>GMSRDRLYTWAGLWRSPSSSWEALRLEDDQAESQLRAPDERSGLPYQLDYRLRWDADWHLREAVFHVESETGVRKLHLLADGRGHWQDGDGEALPAFDGCLDIDIWPSPFTNTFPIRRLGLADGQRAEIRALYIEA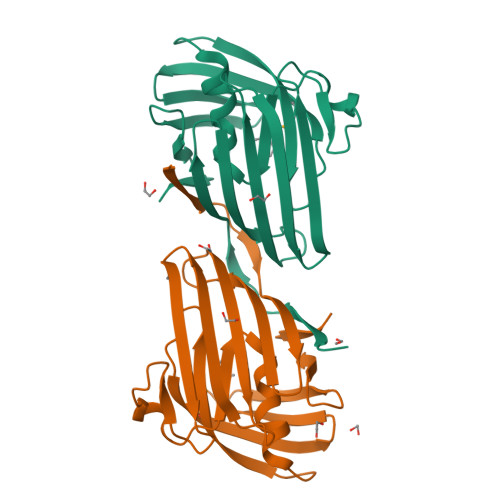PALEPRSMRQAYTRLDASHYLYENLEGSAFKAVLLVDEQGLVIDYPGLFQRL[2x]4-{[(2E)-3,7-dimethylocta-2,6-dien-1-yl]oxy}-7H-furo[3,2-g][1]benzopyran-7-one 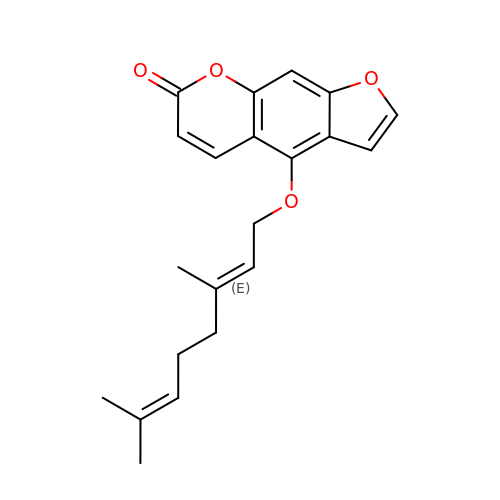| C21 H22 O4 | DBMJZOMNXBSRED-OQLLNIDSSA-N>[2x]SANLPTVLV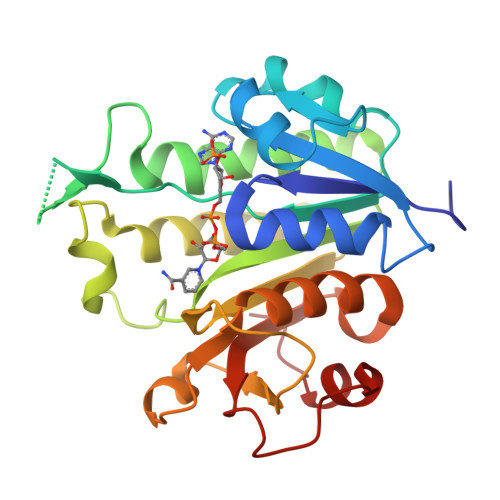TGASGRTGQIVYKKLKEGSDKFVAKGLVRSAQGKEKIGGEADVFIGDITDADSINPAFQGIDALVILTSAVPKMKPGFDPTKGGRPEFIFEDGQYPEQVDWIGQKNQIDAAKVAGVKHIVVVGSMGGTNPDHPLNKLGNGNILVWKRKAEQYLADSGTPYTIIRAGGLLDKEGGVRELLVGKDDELLQTDTKTVPRADVAEVCIQALLFEEAKNKAFDLGSKPEGTSTPTKDFKALFSQVTSRF>SNAMNFNKLKFGATIGIIGGGQLGKMMAQSAQKMGYKVVVLDPSEDCPCRYVAHEFIQAKYDDEKALNQLGQKCDVITYEFENISAQQLKLLCEKYNIPQGYQAIQLLQDRLTEKETLKSAGTKVVPFISVKESTDIDKAIETLGYPFIVKTRFGGYDGKGQVLINNEKDLQEGFKLIETSECVAEKYLNIKKEVSLTVTRGNNNQITFFPLQENEHRNQIL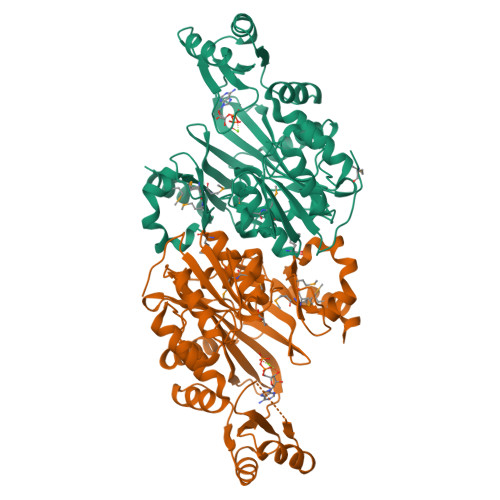FKTIVPARIDKTAEAKEQVNKIIQSIHFIGTFTVEFFIDSNNQLYVNEIAPRPHNSGHYSIEACDYSQFDTHILAVTGQSLPNSIELLKPAVMMNLLGKDLDLLENEFNEHPEWHLHIYGKSERKDSRKMGHMTVLTNDVNQTEQDMYAKFEGSN[2x]> MKGNYVQVYVMLPLDAVSVNNRFEKGDELRAQLRKLVEAGVDGVMVDVWWGLVEGKGPKAYDWSAYKQLFELVQKAGLKLQAIMSFHQCGGNVGDAVNIPIPQWVRDVGTRDPDIFYTDGHGTRNIEYLTLGVDNQPLFHGRSAVQMYADYMTSFRENMKDFLDAGVIVDIEVGLGPAGELRYPSYPQSHGWSFPGIGEFICYDKY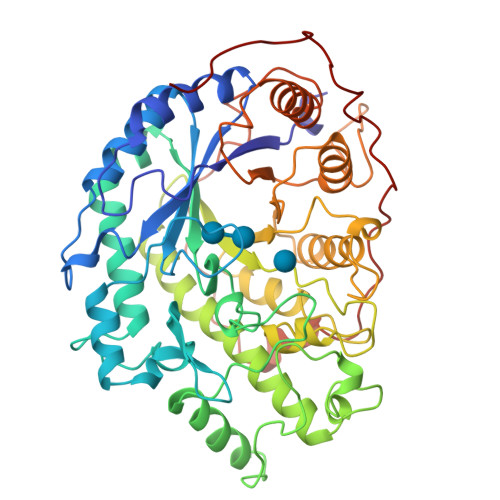LQADFKAAAAAVGHPEWEFPNDAGQYNDTPERTQFFRDNGTYLSEKGRFFLAWYSNNLIKHGDRILDEANKVFLGYKVQLAIKIAGVHWWYKVPSHAAELTAGYYNLHDRDGYRTIARMLKRHRASINFTCAEMRDSEQPPDAMSAPEELVQQVLSAGWREGLNVSCENALPRYDPTAYNTILRNARPHGINQSGPPEHKLFGFTYLRLSNQLVEGQNYVNFKTFVDRMHANLPRDPYVDPMAPLPRSGPEISIEMILQAAQPKIQPFPFQEHTDLPVGPTGGMGGQAEGPTCG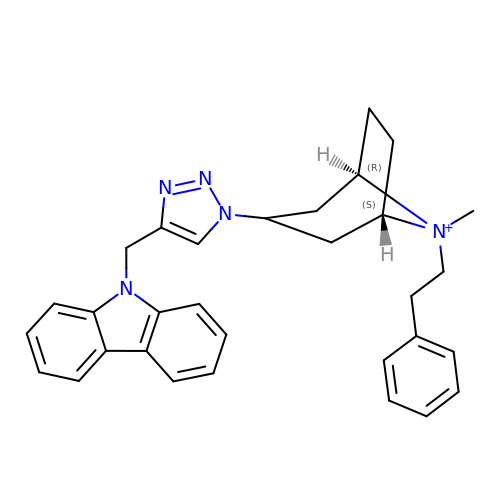9-[[1-[8-methyl-8-(2-phenylethyl)-8-azoniabicyclo[3.2.1]octan-3-yl]triazol-4-yl]methyl]carbazole  | C31 H34 N5 | DLTSAPZJTNDMKP-OYZUSPJKSA-N> SNANINIKKEKVLIPAEVLIQDIPLLKTSFETVRKSRKEIANIIHGNDDRVAVVVGPCSIHDPAAAIEYATKLKEQVKKFHKDILIIMRVYFEKPRTTIGWKGFINDPDLDNSYNINKGLRLARNLLSDLTNMGLPCATEFLDVITPQYFAELITWGAIGARTVESQVHRELASGLSASIGFKNATNGDVQVAVDAVKSATYP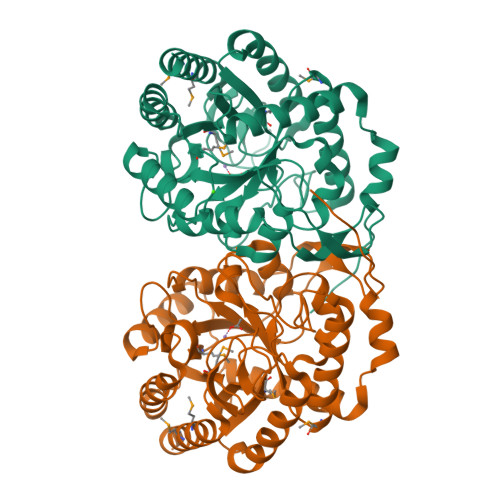HHFLSTTKSGSTAIFATKGNQNGHVILRGGASGPNFSKEHVDDCIAKLKKADINTKVMIDCSHGNSQKDHSKQISVLADICEQIKHSNDIFGVMIESNLVAGNQDINKKPLTYGQSVTDKCVDFEETVKMLEMLAEAVQVRRG>[2x]MAAHHRQNTAGRRKVQVSYVIRDEVEKYNRNGVNALQLDPALNRLFTAGRDSIIRIWSVNQHKQDPYIASMEHHTDWVNDIVLCCNGKTLISASSDTTVKVWNAHKGFCMSTLRTHKDYVKALAYAKDKELVASAGLDRQIFLWDVNTLTALTASNNTVTTSSLSGNKDSIYSLAMNQLGTIIVSGSTEKVLRVWDPRTCAKLMKLKGH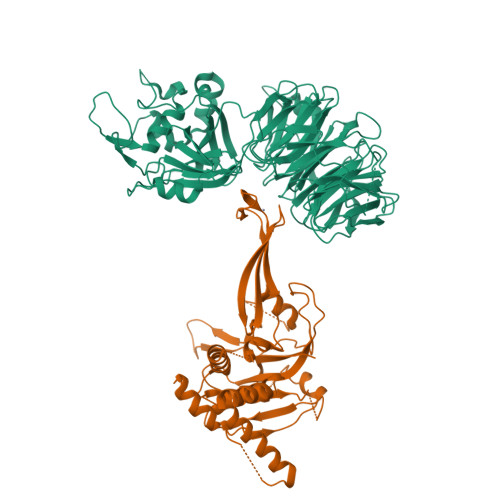TDNVKALLLNRDGTQCLSGSSDGTIRLWSLGQQRCIATYRVHDEGVWALQVNDAFTHVYSGGRDRKIYCTDLRNPDIRVLICEEKAPVLKMELDRSADPPPAIWVATTKSTVNKWTLKGIHNFRASGDYDNDCTNPITPLCTQPDQVIKGGASIIQCHILNDKRHILTKDTNNNVAYWDVLKACKVEDLGKVDFEDEIKKRFKMVYVPNWFSVDLKTGMLTITLDESDCFAAWVSAKDAGFSSPDGSDPKLNLGGLLLQALLEYWPRTHVNPMDEEENEVNHVNGEQENRVQKGNGYFQVPPHTPVIFGEAGGRTLFRLLCRDSGGETESMLLNETVPQWVIDITVDKNMPKFN;>GGSPINCEKRENLLPFVGLNNLGNTCYLNSILQVLYFCPGFKSGVKHLFNIISRKKEALKSLASYELICSLQSLIISVEQLQASFLLNPEKYTDELATQPRRLLNTLRELNPMYEGYLQHDAQEVLQCILGNIQETCQLLKKEEVKNVAENEVKPINKGEEQIGFELVEKLFQGQLVLRTRCLECESLTERREDFQDISVPVQEDELSKVEESSEISPEPKTEMKTLRWAISQFASVERIVGEDKYFCENCHHYTEAERSLLFDKMPEVITIHLKCFAASGLEFDCYGGGLSKINTPLLTPLKLSLEEWSTKPTNDSYGLFAVVMHSGITISSGHYTASVKVTDLNSLEQSLKEYEGKWLLFDDSEVKVTEEKDFLNSLSPSTSPTSTPYLLFYKKL[2x]> MAQLTTESMPF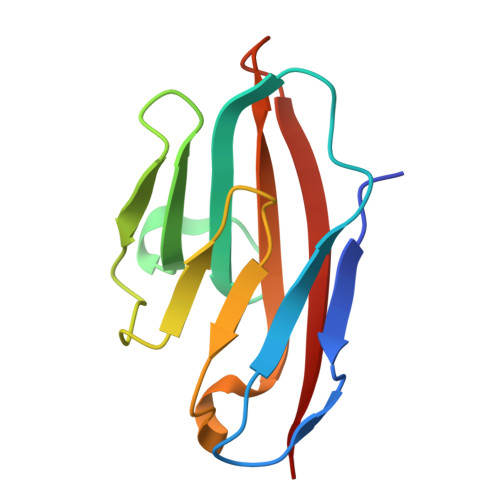NVAEGKEVLLLVHNLPQQLFGYSWYKGERVDGNRQIVGYAIGTQQATPGPANSGRETIYPNASLLIQNVTQNDTGFYTLQVIKSDLVNEEATGQFHVY>[2x]GSHMASGDATDITIYY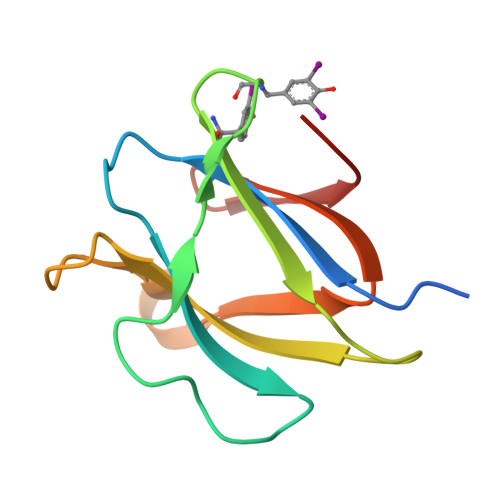KTGWTHPHIHYSLNQGAWTTLPGVPLTKSEYEGYVKVTIEAEEGSQLRAAFNNGSGQWDNNQGRDYDFSSGVHTLADGRILSGTPK> STDASYNADIKEERDAAEGPMAHGIPALNAGALDEARAYATVDSANTDEEVSVAVDVTNLAVVAYRAGSNSYFHAAAPGSSLSHLFSRSSQHTLGFDNTYGDMAQAAGSNRKAIPLGAAALESGIASLNSKNPLARTLMVIIQMLVEAARFRYIQNNVDVSIETQSAFAADAAMISLENNWANLSALVQGSSGGQGTFASSATLQNAEDEPIIVDAVYHPTVAAVLALMLRKAC;> CAAATVRIAGRDGFCADVNGEGQNGAAIILKKCAENDNQLWTLKREATIRSNGGCLTTAAAEQAKAGIYDCTQATAELSAWEIADNGTIINPASSLVLSSGAANSLLDLGVQTNSYASAQGWRTGNETSASVTQISGSAQLCMQAGNGPANLWMSECRAGKAEQQWALLTDKSIRSETNSDNCLTSAADAGPKTILLALCSGPASQRWVFDDDGSILSLYDDKQ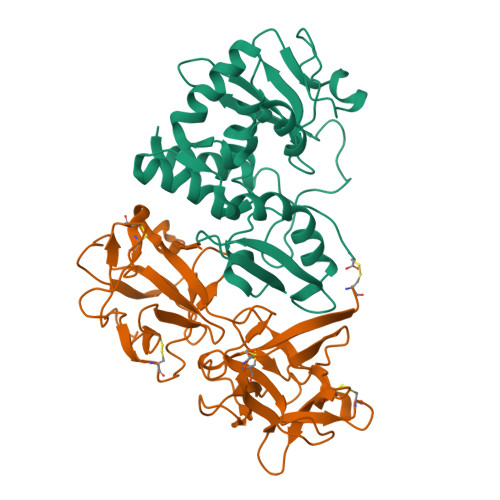MDSEGAAAAAKQIILWWNAAEPNQIWLALF> MNMVMLTIDGKQVQVEKGTTIKKAAEKLGIEIPGLCDDNDLKPFGACRLCVVEDARGNLVASCHTPVREGMVVKTNSPKVLKARRVILELLLSSHNADCFECDKNLHCKLQKYAYELNIRNIRFKGEKRNYEIKDNGPIYYDPNKCILCGKCVRICEEVQHICAIDFASRGFKAYISTPFEKPLLESDCIFCGQCVRVCPTGALAEKTDIERIYEAISDPNKVVVVQVAPAVRVALGEEFGLEPGEIVTGKMVAALKRLGFDKVFDTQFAADMTIVEETAELVERLEKGENFPMFTSCCPSWILAVEKFYPELIPNISTARSPQQIFGAIAKNYYAKKIGVARENMFVVSVMPCIGKKFEATRPEFNNDVDAVLTTRELARMIKESGIDFIKLEEENFDSPLGESTGAAAIFGVTGGVMEAALRTAYSIMTGEELEGDKIEFTAVRGLEGIKEAEVDIKGKKVRIAIANGIGNAKK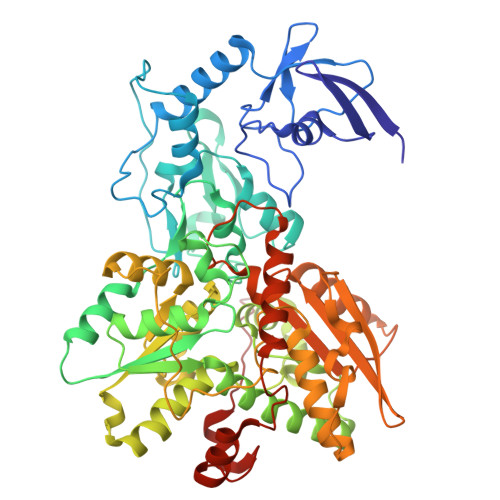LIEKIKSGETKYDFVEVMACPGGCMSGGGQPYTDDPEFRKKRMEGIYKNDRNLPKRKSHENEEVKKVYEEYYEKPCGPKAHEELHTHYHSRKKEY> QGGGRSPSLPTQTCGPWEMKERLGTGGFGYVLRWIHQDTGEQVAIKQCRQELSPKNRERWCLEIQIMKKLNHPNVVSAREVPDGLQKLAPNDLPLLAMEYCEGGDLRKYLNQFENCCGLKEGPIRTLLSDISSALRYLHENRIIHRDLKPENIVLQPGPQRLIHKIID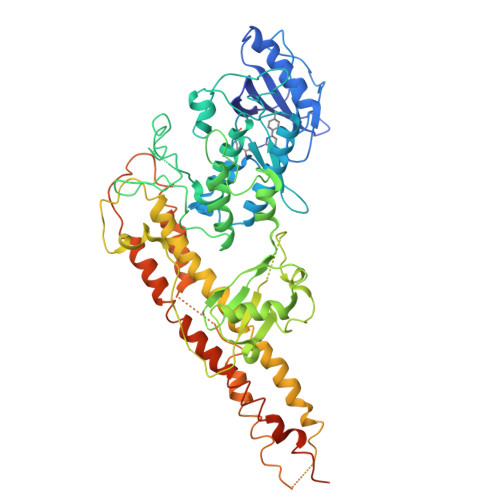LGYAKELDQGELCTEFVGTLQYLAPELLEQKKYTVTVDYWSFGTLAFECITGFRPFLPNWQPVQWHGKVREKSNEHIVVYDDLTGAVKFSSVLPTPNHLSGILAGKLERWLQCMLMWHQRQRGTDPQNPNVGCFQALDSILSLKLLSVMNMVSGRVHTYPVTENENLQNLKSWLQQDTGIPEEEQELLQASGLALNSAQPLTQYVIDCTVIDGRQGEGDLIFLFDNRKTVYEPQISLPAHPESVSIVLQDPKRPLTYTHLRRVWGQIWQTIRALKEDCARLLQGQRTSMVNLLRYNTELSKKKNSMTSECEQLKAKLDFFRSSIQIDLEKYSEQMEFGITSEKLLSAWREMEQAVELCGREREVQALVDKMMALQTDSVDLQRNPLGRKHRGTLDDLEEQARDLYRRLRERPRDQRTPGDSNDMVRLLILAIQSFEKRVILIYDQLSKTVVCKRKALELSPKVKEVMNLMREDEKIVVRRQEKRQQELWNLLKIACSKVRGPVSGSPDS Animal mitochondrial gene expression relies on specific interactions between nuclear-encoded aminoacyl-tRNA synthetases and mitochondria-encoded tRNAs. In this study, we focus on the mitochondrial serylation system, in which a single nuclear-encoded enzyme, mSerRS, charges two distinct mitochondria-encoded mtRNASer isoacceptors. Both, mtRNASer(GCU) and mtRNASer(UGA) have lost the identity-defining long V-arm of the canonical cytosolic tRNASer, and each possesses an unusual secondary structure: While mtRNASer(UGA) adopts a non-canonical cloverleaf fold with extended anticodon stem, mtRNASer(GCU) lacks the entire D-arm33–35, making it the shortest and most degenerated of all human mtRNAs. In contrast to the principle of unimodality found among canonical aaRS-tRNA recognition systems, human mSerRS employs a bimodal recognition mechanism, in which it uses a single binding surface and substrate-specific induced fit to specifically recognize each mtRNASer isoacceptor by orthogonal sets of identity elements.

To understand the molecular basis for mtRNASer(UGA) recognition in human mitochondria, we reconstituted the ternary complex between human mSerRS, the seryl-adenylate analogue 5’-O-[N-(L-seryl)sulfamoyl] adenosine (SerSA), and a stabilized mtRNASer(UGA) transcript, and determined its structure at 3.6 Å resolution using single-particle cryo-EM. Docked across the mSerRS dimer interface, mtRNASer(UGA) establishes interfaces with the active site entrance of subunit 1, the ‘C-tail’ and ‘N-helix’ of subunits 1 and 2, respectively, and the helical arm of subunit 2. Both active sites are occupied by a SerSA ligand, but only one of the two tRNA-binding sites is occupied by a tRNA. The mSerRS-bound mtRNASer(UGA) adopts a non-canonical L-shaped fold, with acceptor-stem-T-arm and anticodon-arm-D-arm domains arranged at an inter-domain angle of ~100°. However, in mtRNASer(UGA) the additional deletion of A9 in the linker between acceptor- and D-stem results in a shift of the entire D-stem by ~3.5 Å (one stacking plane) toward the T-arm. This allows G18 and G19 of the shortened D-loop to form a canonical elbow structure with the T-loop, consistent with earlier chemical probing and NMR data. Thus, mtRNASer(UGA) is bound almost exclusively through its acceptor-T-arm (‘minihelix’) domain, similar to the GCU isoacceptor. As for the mtRNASer(GCU) isoacceptor, mtRNASer(UGA) binding induces a large conformational rearrangement in the motif 2 loop in the entrance to the active site, which inserts residues 334-340 into the major groove of the acceptor stem and forms putative base-specific interactions with C74 of the CCA-end, ‘discriminator base’ (G73), and the first acceptor-stem pair G1:U72.

>[2x]MAASMARRLWPLLTRRGFRPRGGCISNDSPRRSFTTEKRNRNLLYEYAREGYSALPQLDIERFCACPEEAAHALELRKGELRSADLPAIISTWQELRQLQEQIRSLEEEKAAVTEAVRALLANQDSGEVQQDPKYQGLRARGREIRKELVHLYPREAQLEEQFYLQALKLPNQTHPDVPVGDESQARVLHMVGDKPVFSFQPRGHLEIGEKLDIIRQKRLSHVSGHRSYYLRGAGALLQHGLVNFTFNKLLRRGFTPMTVPDLLRGAVFEGCGMTPNANPSQIYNIDPARFKDLNLAGTAEVGLAGYFMDHTVAFRDLPVRMVCSSTCYRAETNTGQEPRGLYRVHHFTKVEMFGVTGPGLEQSSQLLEEFLSLQMEILTELGLHFRVLDMPTQELGLPAYRKFDIEAWMPGRGRFGEVTSASNCTDFQSRRLHIMFQTEAGELQFAHTVNATACAVPRLLIALLESNQQKDGSVLVPPALQSYLGTDRITAPTHVPLQYIGPNQPRKPGLPGQPAVS> QFTDSCLRCICK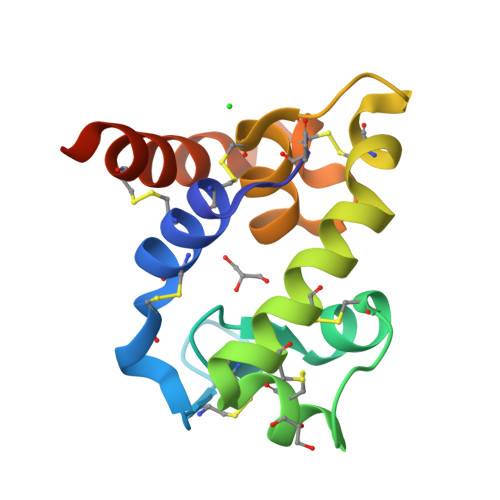VEGCDSQIGKCGMDVGSLSCGPYQIKKPYWIDCGKPGGGYESCTKNKACSETCVRAYMKRYGTFCTGGRTPTCQDYARIHNGGPRGCKSSATVGYWNKVQKCLRGTHHHHHH>[3x]MRCVGISNRDFVEGLSATGWVDVVLEHGSCVTTMAKDKPTLDIELLKTEVTNPAILRKLCIEAKISNTTTDSRCPTQGEATLVEEQDTNFVCRRTFVDRGWGNGCGLFGKGSLITCAKFKCVTKLEGKIVQYENLKYSVIVTVHTGDQHQVGNETTEHGTTATITPQAPTSEIQLTDYGALTLDCSPRTGLDFNEMVLLTMKEKSWLVHKQWFLDLPLPWTSGASTSQETWNRQDLLVTFKTAHAKKQEVVVLGSQEGAMHTALTGATEIQTSGTTTIFAGHLKCRLKMDKLTLKGVSYVMCTGSFKLEKEVAETQHGTVLVQVKYEGTDAPCKIPFSSQDEKGVIQNGRLITANPIVTDKEKPVN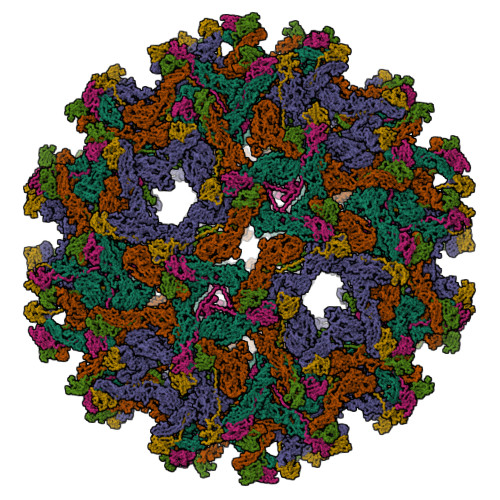IEAEPPFGESYIVVGAGEKALKLSWFKKGSSIGKMFEATARGARRMAILGDTAWDFGSIGGVFTSVGKLVHQIFGTAYGVLFSGVSWTMKIGIGILLTWLGLNSRSTSLSMTCIAVGMVTLYLGVMVQA;>[3x]FHLTTRGGEPHMIVSKQERGKSLLFKTSAGVNMCTLIAMDLGELCEDTMTYKCPRITETEPDDVDCWCNATETWVTYGTCSQTGEHRRDKRSVALAPHVGLGLETRTETWMSSEGAWKQIQKVETWALGHPGFTVIALFLAHAIGTSITQKGIIFILLMLVTPSMA>[6x]MAHHHHHHMATNITFHPGAVTQDERDTLLGQKGCTVWLTGLSASGKSTIATALEQ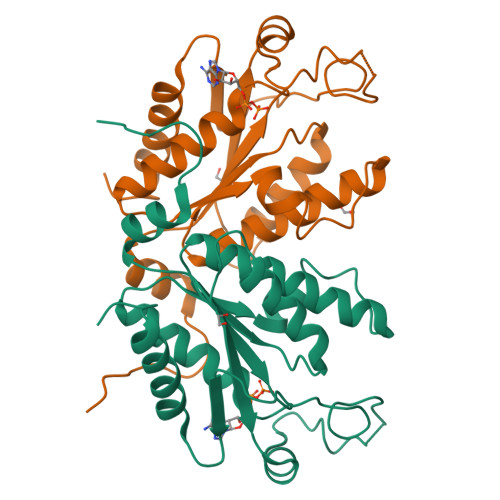HLLHKKLHAYRLDGDNIRFGLNKDLGFDQASRVENIRRIGEVSLLFALSSTISVTAFISPYISDRQLARELHEKHSSAIPFIEVFIDAPLSVVEQRDPKGLYKKARAGEIKDFTGISAPYEAPANPEIHIRTDEVDVAGAVEIITKYLADNGLIPA methyl 2-oxidanylidene-3~{H}-1,3-benzoxazole-6-carboxylate | C9 H7 N O4 | 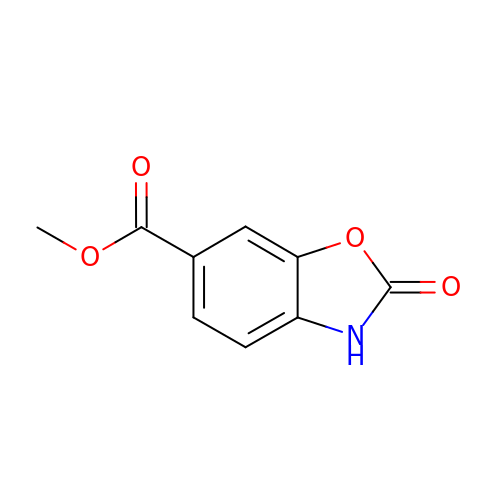FUJBKRLYHYJMNF-UHFFFAOYSA-N> MHHHHHHITSLYKKAGFMKGIYSALMVPYNEDGSINEKGLREIIRYNIDKMKVDGLYVGGSTGENFMISTEEKKRVFEIAIDEAKDSVNLIAQVGSINLNEAVELGKYVTKLGYKCLSAVTPFYYKFDFSEIKDYYETIVRETGNYMIIYSIPFLTGVNMSLSQFGELFENEKIIGVKFTAGDFYLLERVRKAFPDKLIFAGFDEMLLPATVLGVDGAIGSTYNINGIRAKQIFELAKNSKIDEALKIQHTTNDLIEGILSNGLYQTIKEILKLEGVDAGYCRKPMKKISQKQIEFAKELHKKFLKN;> LYKKAGFMKGIYSALMVPYNEDGSINEKGLREIIRYNIDKMKVDGLYVGGSTGENFMISTEEKKRVFEIAIDEAKDSVNLIAQVGSINLNEAVELGKYVTKLGYKCLSAVTPFYYKFDFSEIKDYYETIVRETGNYMIIYSIPFLTGVNMSLSQFGELFENEKIIGVKFTAGDFYLLERVRKAFPDKLIFAGFDEMLLPATVLGVDGAIGSTYNINGIRAKQIFELAKNSKIDEALKIQHTTNDLIEGILSNGLYQTIKEILKLEGVDAGYCRKPMKKISQKQIEFAKELHKKFLK

N-Acetyl-d-neuraminic acid lyase (NanA; EC 4.1.3.3) is also known as sialic acid aldolase. NanA belongs to the class I aldolase family, which is characterized by a triosephosphate isomerase (TIM)-barrel fold and by aldol condensation that proceeds through the formation of a Schiff base intermediate between a conserved lysine residue and the substrate pyruvate. Here, we report 2.32 and 1.76 Å resolution structures of N-acetylneuraminate lyase from F. nucleatum in two forms: ligand-free and with ligand bound as a pyruvate Schiff base. Sequence alignment showed that FnNanA contains conserved catalytic sites (Lys161 and Tyr133) and the conserved specific substrate (Neu5Ac) binding motif GXXGE.

The crystals of ligand-bound FnNanA with a pyruvate Schiff base intermediate belonged to space group P21212 and diffracted to 1.76 Å resolution. The two monomers that were identified appear to form a tetramer with a similar monomer arrangement to those in sialic acid aldolases from other species. The structure has 0.17% Ramachandran outliers. One residue, Lys267 of chain B, is present in the disallowed region; the electron density for this residue is not well defined. All residues were modelled into electron density, except for Tyr108 and Lys109 of chain B in ligand-bound FnNanA with a pyruvate Schiff base and the residues at the N-termini of all monomers. The observed electron-density map for ligand-bound FnNanA with a pyruvate Schiff base in chain A clearly showed that the N∊ atom of Lys161 is conjugated as a Schiff base to the C2 atom of pyruvate. The carboxylate group of the pyruvate makes hydrogen bonds to the backbone N atom of Ser44 and to the hydroxyl group of Thr45. In addition, the Tyr133 side chain makes a hydrogen bond to the hydroxyl group of Ser44 and a conserved water molecule. Tyr133 lies almost parallel to the Schiff base intermediate and is engaged in hydrogen bonding for the Schiff base reaction. The overall architecture of the ligand-bound FnNanA with a pyruvate Schiff base is similar to that of ligand-free FnNanA.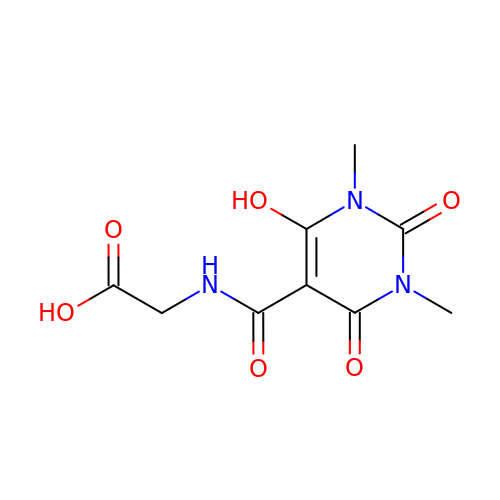(6-hydroxy-1,3-dimethyl-2,4-dioxo-1,2,3,4-tetrahydropyrimidine-5-carbonyl)glycine | C9 H11 N3 O6 | FFGCBWXERBBRBA-UHFFFAOYSA-N>[3x]GHMWPSAKFIDGRVAFSRMPAERELDEVARDF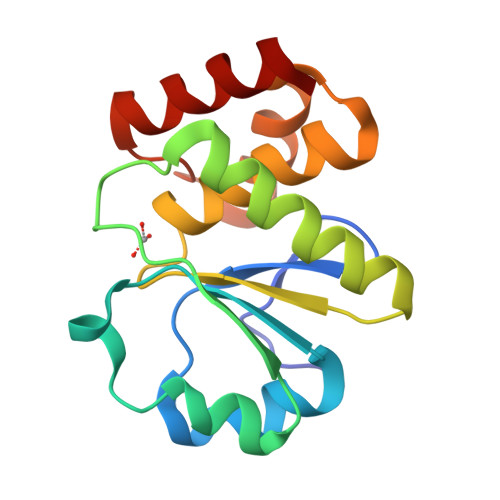DAVVVLVEDYELPYSLDEWEKRGVEVLHGPIPDFTAPSVEQLLEILRWIEERVREGKKVLIHCMGGLGRSGTVGVAWLMYSRGLSLREALMEVRRKRPGAVETQEQMEVLKELEERI propyl 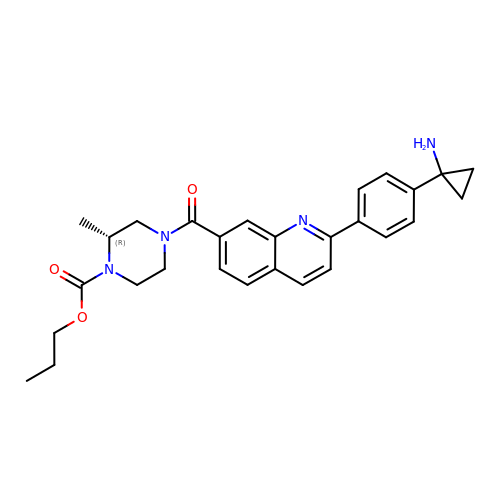(2~{R})-4-[2-[4-(1-azanylcyclopropyl)phenyl]quinolin-7-yl]carbonyl-2-methyl-piperazine-1-carboxylate | C28 H32 N4 O3 | LQPPQWZUQVJLGH-LJQANCHMSA-N>GS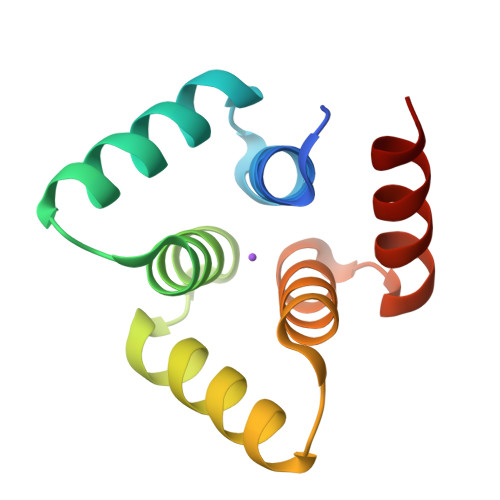SMGKSPTEVLLELIAEASGTTREEVKEKFLKELRKGKSPTEVLLELIAEASGTTKEEVKEKFLKELSFGKSPTEVLLELIAEASGTTKEEVKKKFWKELSL[4x]>MNNLYRDLAPVTEAAWAEIELEAARTFKRHIAGRRVVDVSDPGGPVTAAVSTGRLIDVKAPTNGVIAHLRASKPLVRLRVPFTLSRNEIDDVERGSKDSDWEPVKEAAKKLAFVEDRTIFEGYSAASIEG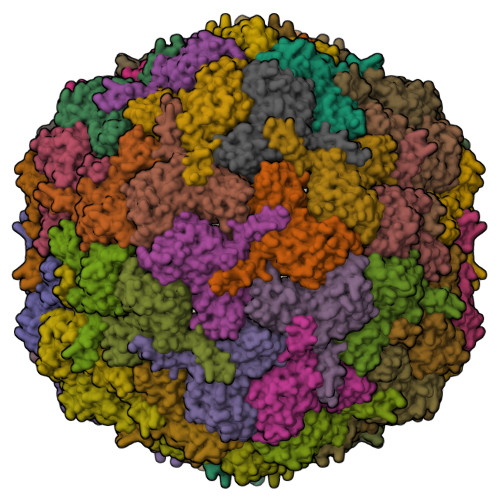IRSASSNPALTLPEDPREIPDVISQALSELRLAGVDGPYSVLLSADVYTKVSETSDHGYPIREHLNRLVDGDIIWAPAIDGAFVLTTRGGDFDLQLGTDVAIGYASHDTDTVRLYLQETLTFLCYTAEASVALSH[60x]>[3x]MFQQLSARLQEAIGRLRGRGRITEEDLKATLREIRRALMDADVNLEVTRDFVERVREEALGKQVLESLTPAEVILATVYEALKEALGGEARLPVLKDRNLW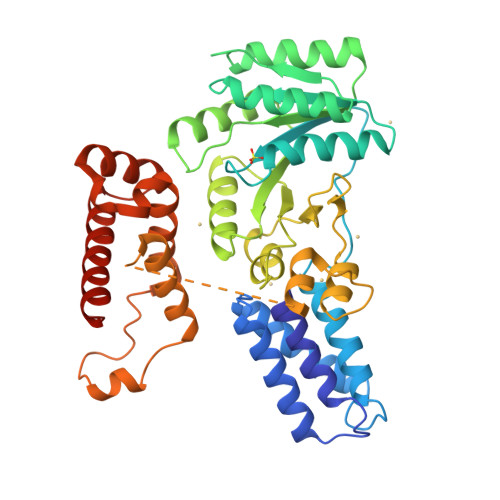FLVGLQGSGKTTTAAKLALYYKGKGRRPLLVAADTQRPAAREQLRLLGEKVGVPVLEVMDGESPESIRRRVEEKARLEARDLILVDTAGRLQIDEPLMGELARLKEVLGPDEVLLVLDAMTGQEALSVARAFDEKVGVTGLVLTKLDGDARGGAALSARHVTGKPIYFAGVSEKPEGLEPFYPERLAGRILGMGDVASLAEKVRAAGLEAEAPKSAKELSLEDFLKQMQNLKRLGPFSEILGLLPGVPQGLKVDEKAIKRLEAIVLSMTPEERKDPRILNGSRRKRIAKGSGTSVQEVNRFIKAFEEMKALMKSLEKKKGRGLM> GGGRPTEIENINPNVYDRIKERVLTANEEDENVPDPFDKREIFDLIRNINDPEHPLTLEELHVVQEDLIRINDSQNSVHISFTPTIPHCSMATLIGLS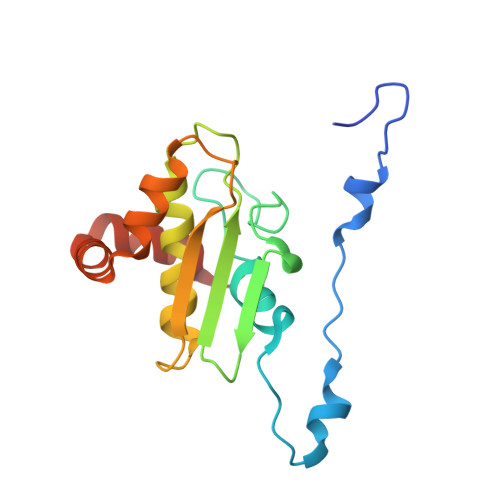IRVKLLRSLPPRFKVTVEITPGTHASELAVNKQLADKERVAAALENNHLAEVINQCIAAKG>[4x]MVAENQPGHIDQIKQTNAGAVYRLIDQLGPVSRIDLSRLAQLAPASITKIVHEMLEAHLVQELEIKEAGNRGRPAVGLVVETEAWHYLSLRISRGEIFLALRDLSSKLVVEESQELALKDDLPLLDRIISHI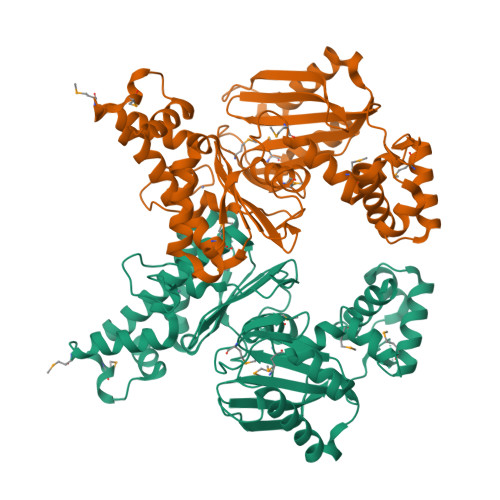DQFFIRHQKKLERLTSIAITLPGIIDTENGIVHRMPFYEDVKEMPLGEALEQHTGVPVYIQHDISAWTMAEALFGASRGARDVIQVVIDHNVGAGVITDGHLLHAGSSSLVEIGHTQVDPYGKRCYCGNHGCLETIASVDSILELAQLRLNQSMSSMLHGQPLTVDSLCQAALRGDLLAKDIITGVGAHVGRILAIMVNLFNPQKILIGSPLSKAADILFPVISDSIRQQALPAYSQHISVESTQFSNQGTMAGAALVKDAMYNGSLLIRLLQG>[2x]GPGSRLNDELLGKVVSVVSATERTEWYPALVISPSCNDDITVKKDQCLVRSFIDSKFYSIARKDIKEVDILNLPESELSTKPGLQKASIFLKTRVVPDNWKMDISEILESSSSDDEDGPAEENDEEKEKEAKKTEEEVPEEELDPEERDNFL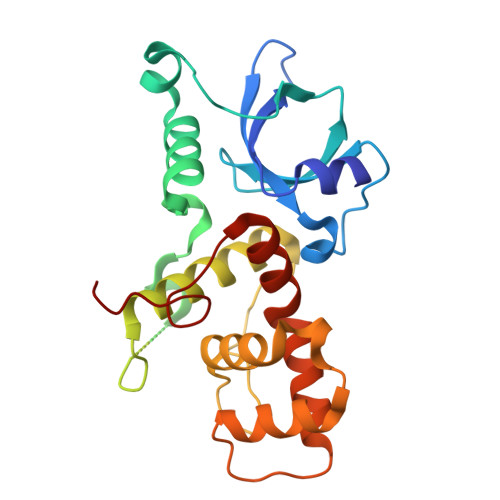QQLYKFMEDRGTPINKPPVLGYKDLNLFKLFRLVYHQGGCDNIDSGAVWKQIYMDLGIPILNSAASYNVKTAYRKYLYGFEEYCRSANIQFRTVHHHEPKV> AAKGGTVKAASGFNAAEDAQTLRKAMKGLGTDEDAIINVLAYRSTAQRQEIRTAYKTTIGRDLMDDLKSELSGNFEQVILGMMTPTVLYDVQELRKAMKGAGTDEGCLIEILASRTPEEIRRINQTYQLQYGRSLEDDIRSDTSFMFQRVLVSLSAGGRDESNYLDDALMRQDAQDLYEAGEKKWGTDEVKFLTVLCSRNRNHLLHVFDEYKRIAQKDIEQSIKSETSGSFEDALLAIVKCMRNKSAYFAERLYKSMKGLGTDDDTLIRVMVSRAEIDMLDIRANF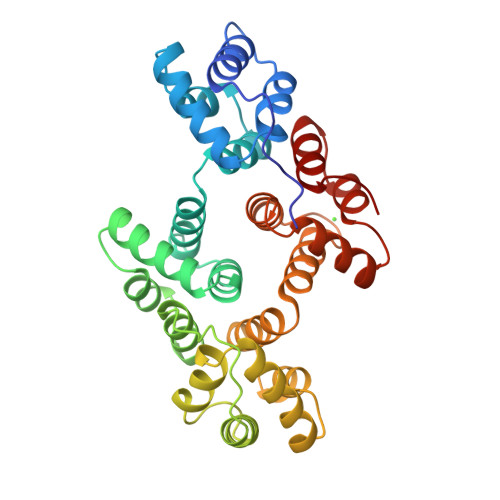KRLYGKSLYSFIKGDTSGDYRKVLLILCGGDD>[4x]MKVGVVGTGFVGSTAAFALVLRGSCSELVLVDRDEDRAQAEAEDIAHAAPVSHGTRVWHGGHSELADAQVVILTAGANQKPGESRLDLLEKNADIFRELVPQITRAAPDAVLLVTSNPVDLLTDLATQLAPGQPVIGSGTVLDSARFRHLMAQHAGVDGTHAHGYVLGEHGDSEVLAWSSAMVAGMPVADFMQAQNL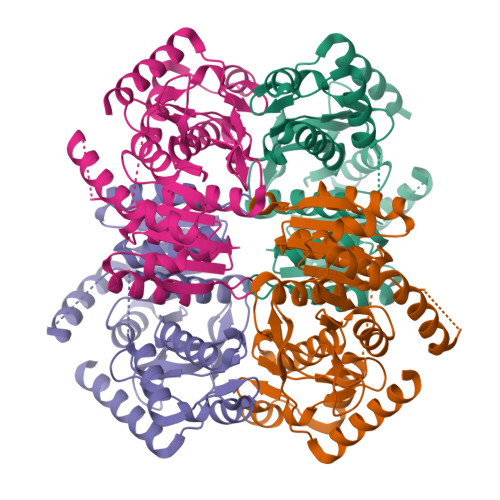PWNEQVRAKIDEGTRNAAASIIEGKRATYYGIGAALARITEAVLRDRRAVLTVSAPTPEYGVSLSLPRVVGRQGVLSTLHPKLTGDEQQKLEQSAGVLRGFKQQLGL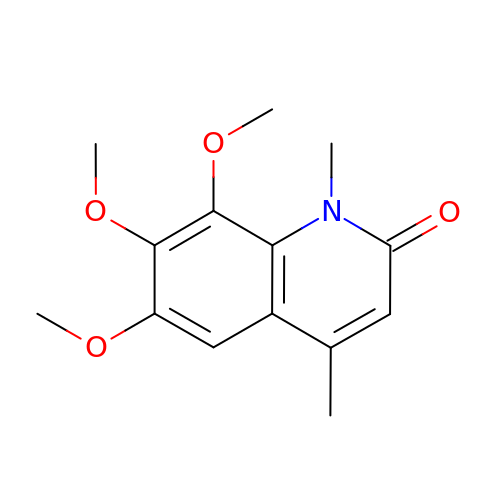6,7,8-trimethoxy-1,4-dimethylquinolin-2(1H)-one | C14 H17 N O4 | QKOJIFYKROBOKN-UHFFFAOYSA-N N-[(1-CHLORO-4-HYDROXYISOQUINOLIN-3-YL)CARBONYL]GLYCINE 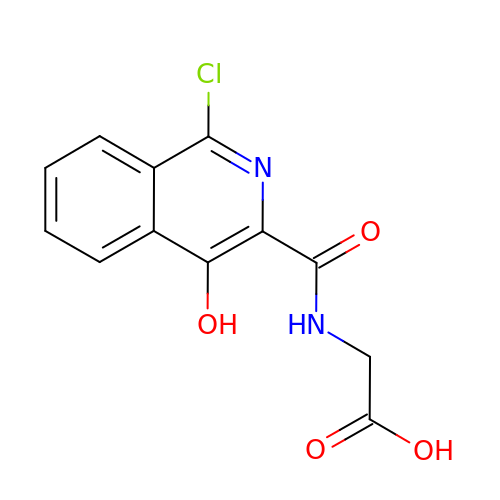| C12 H9 Cl N2 O4 | OUQVKRKGTAUJQA-UHFFFAOYSA-N>XETEKLIRE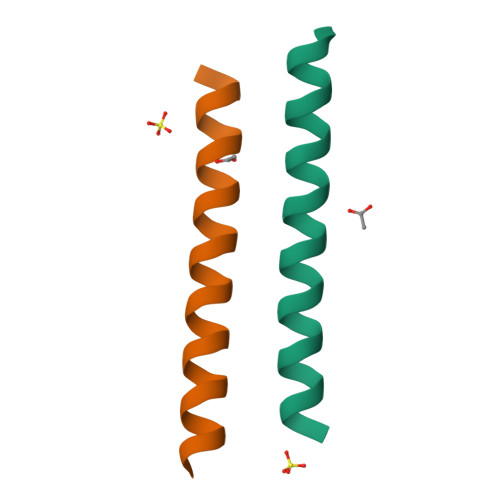KDEELRRMQEMLHKIQKQMKENX[2x]> MNTFHVDFAPNTGEIFAGKQPGDVTMFTLTMGDTAPHGGWRLIPTGDSKGGYMISADGDYVGLYSYMMSWVGIDN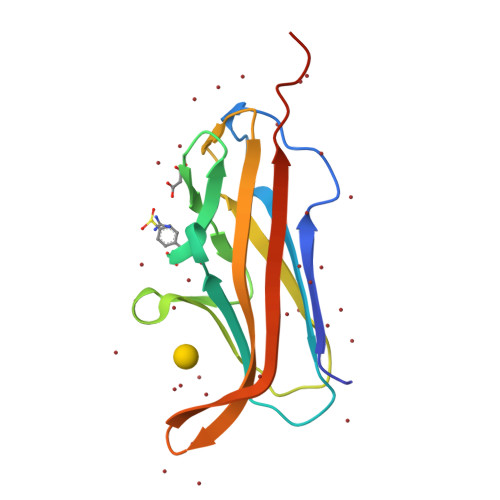NWYINDDSPKDIKDHLYVKAGTVLKPTTYKFTGRVEEYVFDNKQSTVINSKDVSGEVTVKQGLEHHHHHH>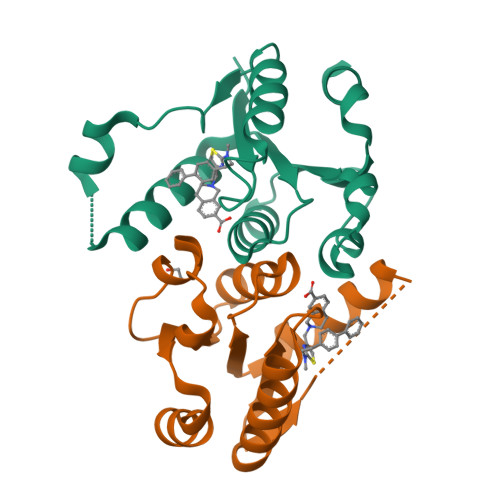MRPALYFCGSIRGGREDRTLYERIVSRLRRFGTVLTEHVAAAELGARGEEAAGGDRLIHEQDLEWLQQADVVVAEVTQPSLGVGYELGRAVAFNKRILCLFRPQSGRVLSAMIRGAADGSRFQVWDYEEGEVEALLDRYFEADPLEENLYFQ[2x]> GUGUGCCCGGCAUGGGUGCAGUCUAUAGGGUGAGAGUCCCGAACUGUGAAGGCAGAAGUAACAGUUAGCCUAACGCAAGGGUGUCCGUGGCGACAUGGAAUCUGAAGGAAGCGGACGGCAAACCUUCGGUCUGAGGAACACGAACUUCAUAUGAGGCUAGGUAUCAAUGGAUGAGUUUGCAUAACAAAACAAAGUCCUUUCUGCCAAAGUUGGUACAGAGUAAAUGAAGCAGAUUGAUGAAGGGAAAGACUGCAU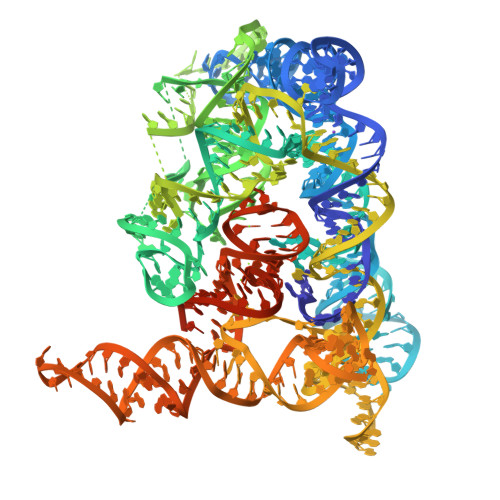UCUUACCCGGGGAGGUCUGGAAACAGAAGUCAGCAGAAGUCAUAGUACCCUGUUCGCAGGGGAAGGACGGAACAAGUAUGGCGUUCGCGCCUAAGCUUGAACCGCCGUAUACCGAACGGUACGUACGGUGGUGUGAGAGGAGUUCGCUCUACUCUAU Glutathione transferases (GSTs) constitute a superfamily of multifunctional proteins widely distributed in nature and they are found in both eukaryotic and prokaryotic organisms. The main role of GSTs is the cellular detoxification of several xenobiotic and endogenous compounds, including drugs. Xi class GSTs form a distinct group of GST enzymes endowed with glutathionyl-hydroquinone reductase activity and show homology with the Omega class GSTs. The present work describes the cloning, expression, purification, crystallization, and structure determination of NmGHR, a GST of the Xi class from the extreme haloalkaliphilic archaeon Natrialba magadii ATCC 43099.

NmGHR was crystallized under high salt conditions and diffraction data were collected to 2.6 Å resolution. NmGHR displays the canonical GST fold with a N-terminal thioredoxin-like domain and a C-terminal all-helical domain. The protein backbone and relative orientation of the monomers in the dimeric assembly is remarkably well conserved between archaeal NmGHR and it mesophilic counterparts. Furthermore these values are comprised between 1.2 and 1.78 Å when directly superposing the dimers. These observations suggests that not only the canonical GST fold is perfectly compatible with halotolerance but also the quaternary structure, posing this class of enzymes as one of the most structurally conserved when comparing halophilic proteins to their mesophilic counterparts. As expected, NmGHR is characterized by an extremely high content of negatively charged residues which are evenly distributed throughout the surface of the protein. An interesting feature of NmGHR structure is that the histidine-tag present at the N-terminus of the protein chain to aid purification is ordered and visible. We could model in the electron density the complete tag including the initial methionine of chain A, and almost completely also of chain B. As shown in Figure 5A, the tag sits along a wide cleft between the N-terminal and C-terminal domains of NmGHR. However, it may also be noted that, under this framework, the amino-terminal group of γ-Glu-Cys is as close as 1.4 Å from the side chain of the methionine (-6) that precedes the hexa-histidine-tag. This suggests that, in our experimental conditions, the histidine-tag partly occludes the enzyme’s G-site, possibly explaining why our soaking or co-crystallization experiments failed to recover γ-Glu-Cys in the crystals. Therefore the absence of S-glutathionyl-hydroquinone reductase activity that we detected with the classical substrate for Xi class GSTs, i.e., benzoquinone, might be due to the position occupied by the tag in high salt conditions.

>[2x]MHHHHHHMNMLVDGEWRTDAHELTAGDGSFERQATTFRNWVQDDSDARFQPEAGRYHLYVSYACPWAHRTLVTRTLKGLEDAISVSVVDPYRAEDGWQFTPEKEGCTHDHVHDVDYLRELYVRAAPDVTCRVTVPVLWDTEEDTIVNNESEEIMRMFDTEFDEFADHTVDLYPEGYQEKVDQIIDNIYEPINNGVYRAGFATEQEPYDEAVAELFGALAHWDDVLADQRYLAGDRLTEADIAMFTTLVRFDNVYHTHFMCNVQYIREFDNLWPYLRDLYQTHGIAETVEMDHITEHYYTTHPDVNPHRIVARGPDLDFEAPHSRDELAGEPPAALVSSAGR> DREEAAFLAASILIQHAHEQGKDDRELEKILEIAIRILEKNGVDREEAAFLAASILIQHAHEQGKDDRELEKILEIAIRILEKNGVDREEAAFLAASILIQHAHEQGKDDRELEKILEIAIR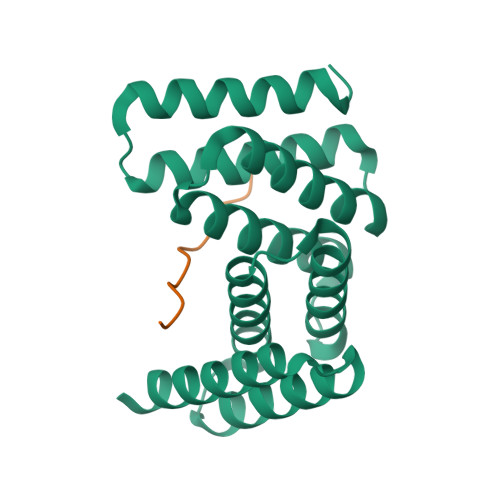ILEKNGVDREEAAFLAASILIQHAHEQGKDDRELEKILEIAIRILEKNGV;> LRPLRPLRPLRP> MILHALTQYYQRKAESDGGIAQEGFENKEIPFIIVIDKQGNFIQLEDTRELKVKKKVGRTFLVPKGLGRSGSKSYEVSNLLWDHYGYVLAYAGEKGQEQADKQHASFTAKVNELKQALPDDAGVTAVAAFLSSAEEKSKVMQAANWAECAKVKGCNLSFRLVDEAVDLVCQSKAVREYVSQANQTQSDNAQKGICLVTGKAAPIARLHNAVKGVNA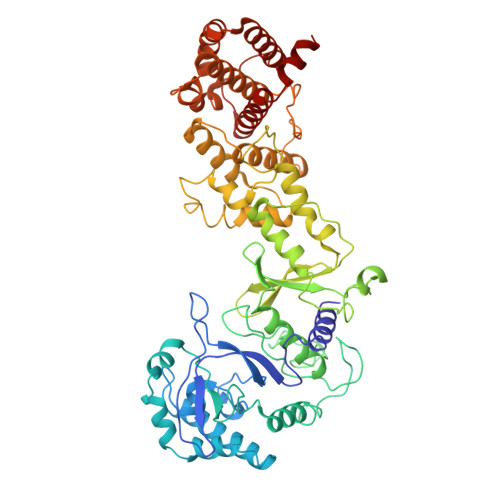KPAPFASVNLSAFESYGKEQGFAFPIGEQAMFEYTTALNTLLAGENRFRIGDVTTVCWGAKRTPLEESLASMINGGGKDNPDAHIDAVKALYKSLYNGQYCKPDGEDKFYLLGLSPNSARIVVRFWHETTVAALSESIAAWYDDLQMVRGENSPYPEYMPLPRLLGNLVLDGKMENLPSDLIAQITDAALNNRVLPVSLLQAALRRNKAEQKITYGRASLLKAYINRAIRAGRLKNMKELTMGLDRNRQDIGYVLGRLFAVLEKIQAEANPGLNATIADRYFGSASSTPIAVFGTLMRLLPHHLNKLEFEGRAVQLQWEIRQILEHCQRFPNHLNLEQQGLFAIGYYHETQFLFTKDALKNLFNEA>GSGSGAPMTSIHFVVHPLPGTEDQLNDRLREVSEKLNKYNLNSHPPLNVLEQATIKQCVVGPNHAAFLLEDGRVCRIGFSVQPDRLELGKPDNNDGSKLNSNSGAGRTSRPGRTSDSPWFLSGSETLGRLAGNTLGSRWSSGVGGSGGGSSGRSSAGARDSRRQTRVIRTGRDRGSGLLGSQPQPVIPASVIPEELISQAQVVLQGKSRSVIIRELQRTNLDVNLAVNNLLSRDDEDGDDGDDTASESYLPGEDLMSLLDADIHSAHPSVIIDADAMFSEDISYFGYPSFRRSSLSRLGSSRVLLLPLERDSELLRERESVLRLRERRWLDGASFDNERGSTSKEGEPNLDKKNTPVQSPVSLGEDLQWWPDKDGTKFICIGALYSELLAVSSKGELYQWKWSESEPYRNAQNPSLHHPRATFLGLTNEKIVLLSANSIRATVATENNKVATWVDETLSSVASKLEHTAQTYSELQGERIVSLHCCALYTCAQLENSLYWWGVVPFSQRRKMLEKARAKNKKPKSSAGISSMPNITVGTQVCLRNNPLYHAGAVAFSISAGIPKVGVLMESVWNMNDSCRFQLRSPESLKNMEKASKTTEAKPESKQEPVKTEMGPPPSPASTCSDASSIASSASMPYKRRRSTPAPKEEEKVNEEQWSLREVVFVEDVKNVPVGKVLKVDGAYVAVKFPGTSSNTNCQNSSGPDADPSSLLQDCRDLRIDELQVVKTGGTPKVPDCFQRTPKKLCIPEKTEILAVNVDSKGVHAVLKTGNWVRYCIFDLATGKAEQENNFPTSSIAFLGQNERNVAIFTAGQESPIILRDGNGTIYPMAKDCMGGIRDPDWLDLPPISSLGMGVHSLINLPANSTIKKKAAVIIMAVEKQTLMQHILRCDYEACRQYLMNLEQAVVLEQNLQMLQTFISHRCDGNRNILHACVSVCFPTSNKETKEEEEAERSERNTFAERLSAVEAIANAISVVSSNGPGNRAGSSSSRSLRLREMMRRSLRAAGLGRHEAGASSSDHQDPVSPPIAPPSWVPDPPAMDPDGDIDFILAPAVGSLTTAATGTGQGPSTSTIPGPSTEPSVVESKDRKANAHFILKLLCDSVVLQPYLRELLSAKDARGMTPFMSAVSGRAYPAAITILETAQKIAKAEISSSEKEEDVFMGMVCPSGTNPDDSPLYVLCCNDTCSFTWTGAEHINQDIFECRTCGLLESLCCCTECARVCHKGHDCKLKRTSPTAYCDCWEKCKCKTLIAGQKSARLDLLYRLLTATNLVTLPNSRGEHLLLFLVQTVARQTVEHCQYRPPRIREDRNRKTASPEDSDMPDHDLEPPRFAQLALERVLQDWNALKSMIMFGSQENKDPLSASSRIGHLLPEEQVYLNQQSGTIRLDCFTHCLIVKCTADILLLDTLLGTLVKELQNKYTPGRREEAIAVTMRFLRSVARVFVILSVEMASSKKKNNFIPQPIGKCKRVFQALLPYAVEELCNVAESLIVPVRMGIARPTAPFTLASTSIDAMQGSEELFSVEPLPPRPSSDQSSSSSQSQSSYIIRNPQQRRISQSQPVRGRDEEQDDIVSADVEEVEVVEGVAGEEDHHDEQEEHGEENAEAEGQHDEHDEDGSDMELDLLAAAETESDSESNHSNQDNASGRRSVVTAATAGSEAGASSVPAFFSEDDSQSNDSSDSDSSSSQSDDIEQETFMLDEPLERTTNSSHANGAAQAPRSMQWAVRNTQHQRAASTAPSSTSTPAASSAGLIYIDPSNLRRSGTISTSAAAAAAALEASNASSYLTSASSLARAYSIVIRQISDLMGLIPKYNHLVYSQIPAAVKLTYQDAVNLQNYVEEKLIPTWNWMVSIMDSTEAQLRYGSALASAGDPGHPNHPLHASQNSARRERMTAREEASLRTLEGRRRATLLSARQGMMSARGDFLNYALSLMRSHNDEHSDVLPVLDVCSLKHVAYVFQALIYWIKAMNQQTTLDTPQLERKRTRELLELGIDNEDSEHENDDDTNQSATLNDKDDDSLPAETGQNHPFFRRSDSMTFLGCIPPNPFEVPLAEAIPLADQPHLLQPNARKEDLFGRPSQGLYSSSASSGKCLMEVTVDRNCLEVLPTKMSYAANLKNVMNMQNRQKKEGEEQPVLPEETESSKPGPSAHDLAAQLKSSLLAEIGLTESEGPPLTSFRPQCSFMGMVISHDMLLGRWRLSLELFGRVFMEDVGAEPGSILTELGGFEVKESKFRREMEKLRNQQSRDLSLEVDRDRDLLIQQTMRQLNNHFGRRCATTPMAVHRVKVTFKDEPGEGSGVARSFYTAIAQAFLSNEKLPNLECIQNANKGTHTSLMQRLRNRGERDREREREREMRRSSGLRAGSRRDRDRDFRRQLSIDTRPFRPASEGNPSDDPEPLPAHRQALGERLYPRVQAMQPAFASKITGMLLELSPAQLLLLLASEDSLRARVDEAMELIIAHGRENGADSILDLGLVDSSEKVQQENRKRHGSSRSVVDMDLDDTDDGDDNAPLFYQPGKRGFYTPRPGKNTEARLNCFRNIGRILGLCLLQNELCPITLNRHVIKVLLGRKVNWHDFAFFDPVMYESLRQLILASQSSDADAVFSAMDLAFAIDLCKEEGGGQVELIPNGVNIPVTPQNVYEYVRKYAEHRMLVVAEQPLHAMRKGLLDVLPKNSLEDLTAEDFRLLVNGCGEVNVQMLISFTSFNDESGENAEKLLQFKRWFWSIVEKMSMTERQDLVYFWTSSPSLPASEEGFQPMPSITIRPPDDQHLPTANTCISRLYVPLYSSKQILKQKLLLAIKTKNFGFV[6x]

UBR5 has key roles in stem cell pluripotency, tumor suppression, oncogenesis and other important pathways. We used chemistry and cryo‐electron microscopy (cryo‐EM) to visualize stable mimics of the intermediates along K48-linked Ub chain formation by the human E3, UBR5. The structural data reveal a ≈ 620 kDa UBR5 dimer as the functional unit, comprising a scaffold with flexibly tethered Ub-associated (UBA) domains, and elaborately arranged HECT domains. Our data show how a full-length E3, ubiquitins to be adjoined, E2 and intermediary products guide a feed-forward HECT domain conformational cycle establishing a highly efficient, broadly targeting, K48-linked Ub chain forging machine.

Indeed, an L710D variant at the dSBB interface prevented tetramerization and led to the formation of a catalytically active dimer. Cryo-EM data for the L710D variant, hereafter termed UBR5Dimer, yielded a map allowing the building and refining of a twofold symmetric experimentally derived structure at 2.7 Å resolution. The N-terminal region consists of an interrupted RCC1-like domain (RLD) β-propeller, with UBA (not visible in the map) and dSBB domains inserted in blades 2 and 5, respectively. The central region is primarily α-helical but also embeds the UBR domain that has been proposed to bind substrate N-termini. UBR5’s C-terminal HECT domain initiates with residues not originally annotated as being part of this domain and adopts the L-conformation. The HECT domain L-configuration is stabilized by numerous interactions. Two meandering sequences emanating from the scaffold—which we term domain swap dimerization (DSD, residues 1691–1720) and HECT display (HD, residues 2016–2076) domains—extensively bind the HECT domain. One protomer’s DSD domain contributes to the extensive dimerization interface within the scaffold, while a peptide-like loop projects from the scaffold to bind the C-lobe from one HECT domain. Meanwhile, one side of the HD domain interacts with the α-helical portion of the scaffold, and the other side nestles in a concave surface of the HECT domain N-lobe opposite the E2-binding site. Numerous additional interactions further position UBR5’s HECT domain, including between the central region and HECT domain N-terminus, and between the HECT domain N- and C-lobes.>MKKPNGTNGASSSLEPPPSTFQPLCHPLVEEVSKEVDGYFLQHWNFPNEKARKKFVAAGFSRVTCLYFPKALDDRIHFACRLLTVLFLIDDLLEYMSFEEGSAYNEKLIPISRGDVLPDRSIPVEYIIYDLWESMRAHDREMADEILEPVFLFMRAQTDRTRARPMGLGGYLEYRERDVGKELLAALMRFSMGLKLSPSELQRVREIDANCSKHLSVVNDIYSYE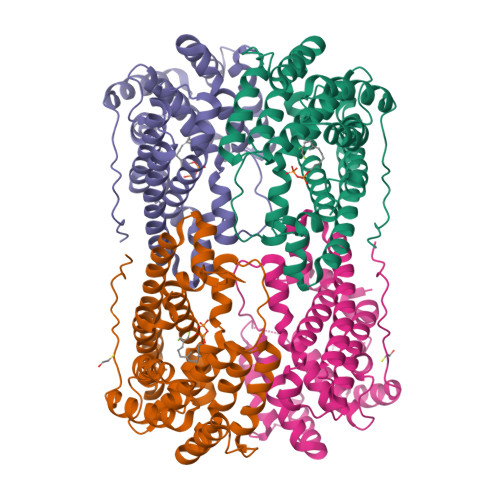KELYTSKTAHSEGGILCTSVQILAQEADVTAEAAKRVLFVMCREWELRHQLLVARLSAEGLETPGLAAYVEGLEYQMSGNELWSQTTLRYSVVVD[4x]> AIETETLVVGAGPGGYVAAIRAAQLGQKVTIVEKGNLGGVCLNVGCIPSKALISASHRYEQAKHSEEMGIKAENVTIDFAKVQEWKASVVKKLTGGVEGLLKGNKVEIVKGEAYFVDANTVRVVNGDSAQTYTFKNAIIATGSRPIELPNFKFSNRILDSTGALNLGEVPKSLVVIGGGYIGIEL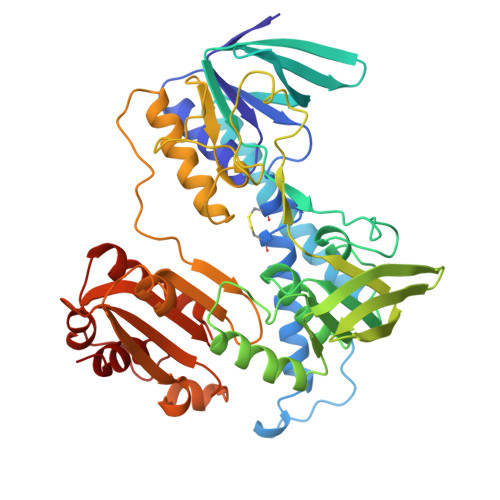GTAYANFGTKVTILEGAGEILSGFEKQMAAIIKKRLKKKGVEVVTNALAKGAEEREDGVTVTYEANGETKTIDADYVLVTVGRRPNTDELGLEQIGIKMTNRGLIEVDQQCRTSVPNIFAIGDIVPGPALAHKASYEGKVAAEAIAGHPSAVDYVAIPAVVFSDPECASVGYFEQQAKDEGIDVIAAKFPFAANGRALALNDTDGFLKLVVRKEDGVIIGAQIIGPNASDMIAELGLAIEAGMTAEDIALTIHAHPTLGEIAMEAAEVAL> MSLLLTIAKEYKRLCQDAKAAQMMTVGTVSNYTTFKKWTTSRKEKNPSLRMRWAMSSKFPIIANKRMLEEAQIPKEHNNVALWEDTEDVSKRDHVLASASCINYWNFCGPCVNNSEVIKEVYKSRFGRLERRKEIMWKELRFTLVDRQRRRVDTQPVEQRLRTGEIKDLQMWTLFEDEAPLASKFILDNYGLVKEMRSKFANKPLNKEVVAH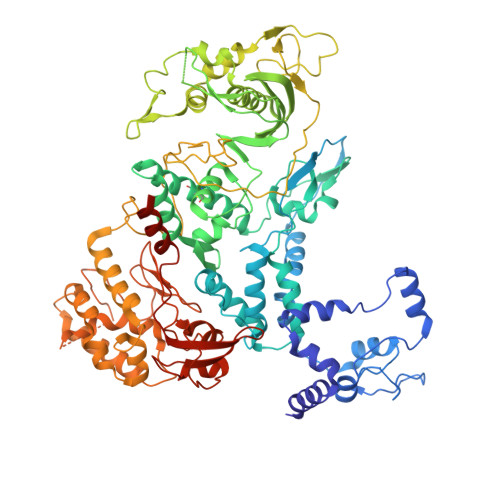MLEKQFNPESRFLPVFGAIRPERMELIHALGGETWIQEANTAGISNVDQRKNDIRAVCRKVCLAANASIMNAKSKLVEYIKSTSMRIGETERKLEELILETDDVSPEVTLCKSALGGQLGKTLSFGPMLLKKISGSGVKVKDTVYIQGVRAVQFEYWSEQEEFYGEYKSATALFSRKERSLEWITIGGGINEDRKRLLAMCMIFCRDGDYFKDAPATITMADLSTKLGREIPYQYVMMNWIQKSEDNLEALLYSRGIVETNPGKMGSSMGIDGSKRAIKSLRAVTIQSGKIDMPESKEKIHLELSDNLEAFDSSGRIVATILDLPSDKKVTFQDVSFQHPDLAVLRDEKTAITKGYEALIKRLGTGDNDIPSLIAKKDYLSLYNLPEVKLMAPLIRPNRKGVYSRVARKLVSTQVTTGHYSLHELIKVLPFTYFAPKQGMFEGRLFFSNDSFVEPGVNNNVFSWSKADSSKIYCHGIAIRVPLVVGDEHMDTSLALLEGFSVCENDPRAPMVTRQDLIDVGFGQKVRLFVGQGSVRTFKRTASQRAASSDVNKNVKKIKMSNARENLYFQ>[2x]ASVSSYHLFRDVAEVTAFRGSLLSWYDQEKRDLPWRRRAEDEMDLDRRAYAVWVSEVMLQQTQVATVINYYTGW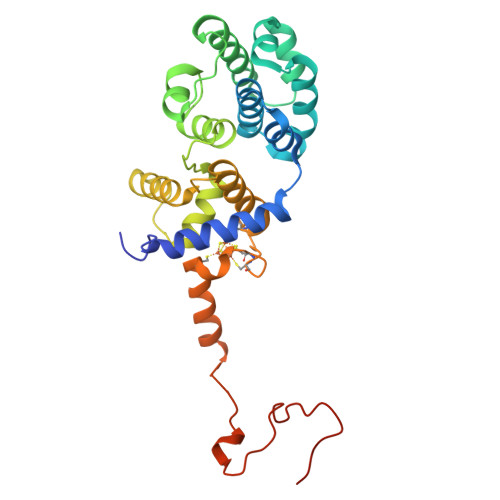MQKWPTLQDLASASLEEVNQLWAGLGYYSRGRRLQEGARKVVEELGGHMPRTAETLQQLLPGVGRYTAGAIASIAFGQATGVVDGNVARVLCRVRAIGADPSSTLVSQQLWGLAQQLVDPARPGDFNQAAMELGATVCTPQRPLCSQCPVESLCRARQRVEQEQLLASGSLSGSPDVEECAPNTGQCHLCLPPSEPWDQTLGVVNFPRKASRK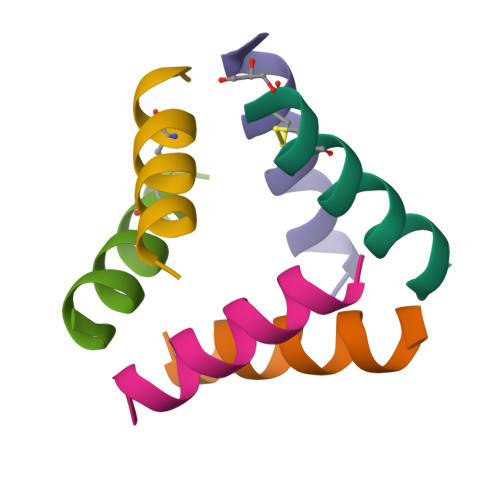>[24x]LKKLCKLLKKLCKLAG>[2x]MQPLFTQERRIFHKKLLDGNILATNNRGVVSNADGSNTRSFNIAKGIADLLHSETVSERLPGQTSGNAFEAICSEFVQSAFEKLQHIRPGDWNVKQVGSRNRLEIARYQQYAHLTALAKAAEENPELAAALGSDYTITPDIIVTRNLIADAEINRNEFLVDENIATYASLRAGNGNMPLLHASISCKWTIRSDRAQNARSEGL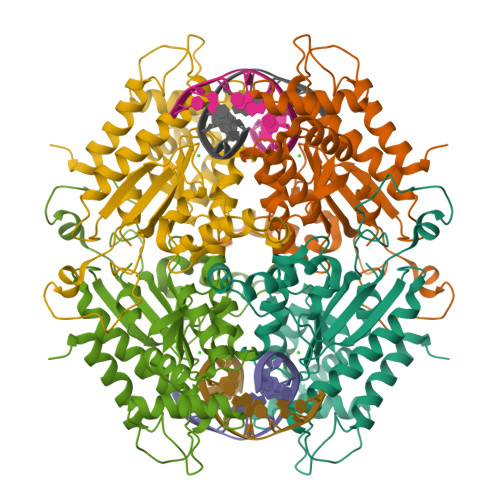NLVRNRKGRLPHIVVVTAEPTPSRISSIALGTGEIDCVYHFALYELEQILQSLNYEDALDLFYIMVNGKRLKDISDLPLDLAV2-IMINOBIOTIN | C10 H17 N3 O2 S | 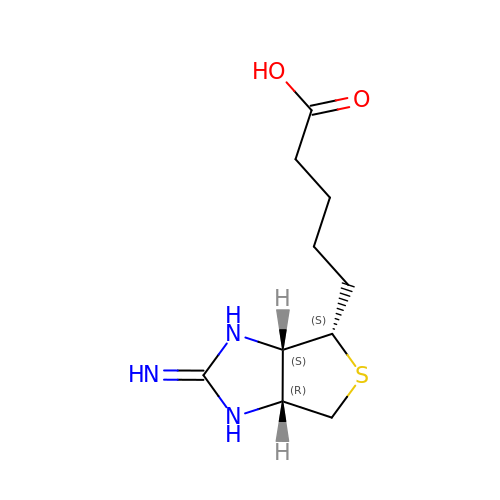WWVANQJRLPIHNS-ZKWXMUAHSA-N>PNFSGNWKIIRSENFEELLKVLGVNVMLRKIAVAAASKPAVEIKQEGDTFYIKTSTTVRTTEINFKVGEEFEEQTVDGRPCKSLVKWESENKMVCEQKLLKGEGPKTSWTRELTNDGELILTMTADDVVCTKVFVR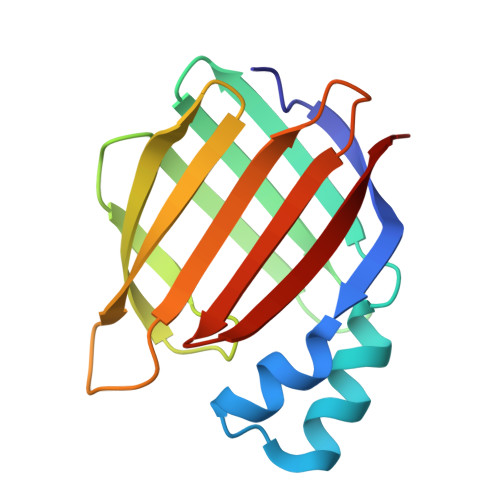E[2x]> MKINRQQYAESYGPTVGDQVRLADTDLWIEVEKDYTTYGDEANFGGGKVLREGMGENGTYTRTENVLDLLLTNALILDYTGIYKADIGVKDGYIVGIGKGGNPDIMDGVTPNMIVGTATEVIAAEGKIVTAGGIDTHVHFINPDQVDVALAN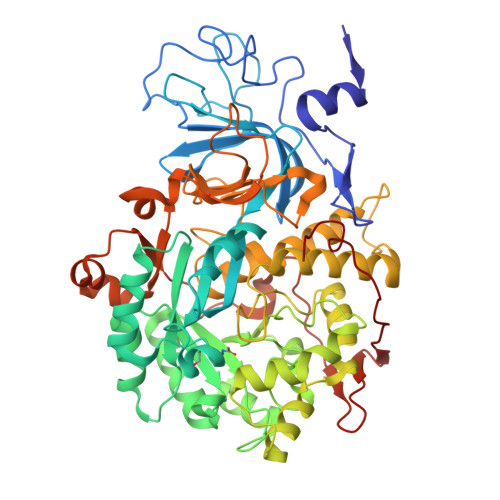GITTLFGGGTGPAEGSKATTVTPGPWNIEKMLKSTEGLPINVGILGKGHGSSIAPIMEQIDAGAAGLKIHEDWGATPASIDRSLTVADEADVQVAIHSDTLNEAGFLEDTLRAINGRVIHSFHVEGAGGGHAPDIMAMAGHPNVLPSSTNPTRPFTVNTIDEHLDMLMVCHHLKQNIPEDVAFADSRIRPETIAAEDILHDLGIISMMSTDALAMGRAGEMVLRTWQTADKMKKQRGPLAEEKNGSDNFRAKRYVSKYTINPAIAQGIAHEVGSIEEGKFADLVLWEPKFFGVKADRVIKGGIIAYAQIGDPSASIPTPQPVMGRRMYGTVGDLIHDTNITFMSKSSIQQGVPAKLGLKRRIGTVKNCRNIGKKDMKWNDVTTDIDINPETYEVKVDGEVLTCEPVKELPMAQRYFLF>[2x]SRGKGNFSACTHSFGGTRDHDVVEEFIGNIETYKDVEGISDENALKGISLLFYGMASTWWQGVRKEATTWKEAIALIREHFSPTKPAYQIYMEFFQNKQDDHDPIDT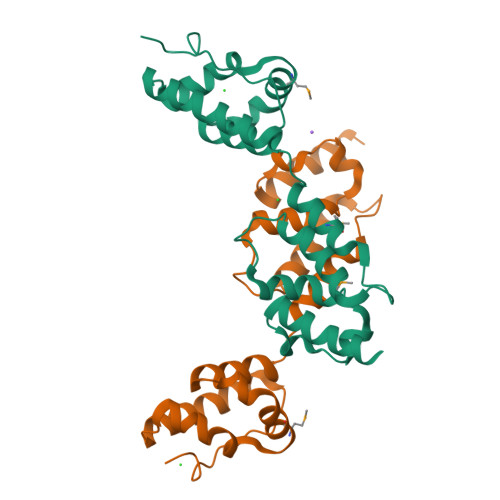FVIQKRALLAQLPSGRHDEETELDLLFGLLNIKYRKHISRHSVHTFKDLLEQGRIIEHNNPLE>SMS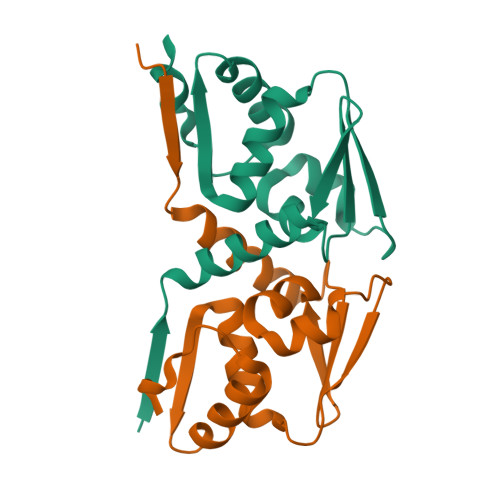VFAYESSVHSTNVLLSLNDQRKKDVLCDVTIFVEGQRFRAHRSVLAACSSYFHSRIVGQADGELNITLPEEVTVKGFEPLIQFAYTAKLILSKENVDEVCKCVEFLSVHNIEESCFQFLKF[4x]>[2x]HMTALTLPEDIRQQEPSALLYTLVSAYLEHTAQTGDESLSCLSDDQHTLTAFCYLDSQVEEGGFVQLIASGYGEYIFRNPLA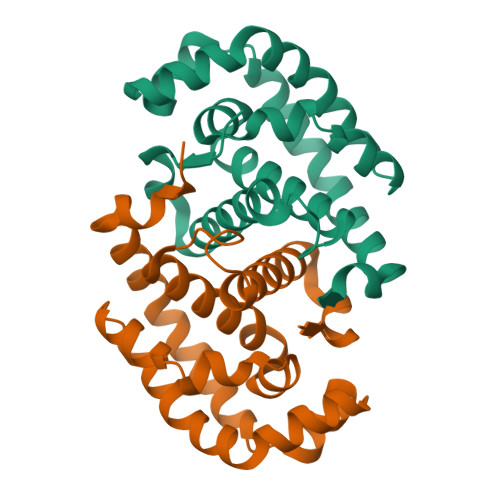DSLRRWKIKAVPKVLDKAKALYEQHGKTIETLADGGADIPSLRKQFPEFEEWDGAYYEAAEQDLPLLAEHIQSNWETFAHIGQA>KNNPDPTIYPVLDWNDIKFQDVIGEGNFGQVLKARIKKDGLRMDAAIKRMKEYASKDDHRDFAGELEVLCKLGHHPNIINLLGACEHRGYLYLAIEYAPHGNLLDFLRKSRVLETDPAFAIANSTASTLSSQQLLHFAADVARGMDYLSQKQFIHRDLAARNILVGENYVAKIADFGLSRGQEVYVKKTMGRLPVRWMAIESLNYSVYTTNSDVWSYGVLLWEIVSLGGTPYCGMTCAELYEKLPQGYRLEKPLNCDDEVYDLMRQCWREKPYERPSFAQILVSLNRMLEERKTYVNTTLYEKF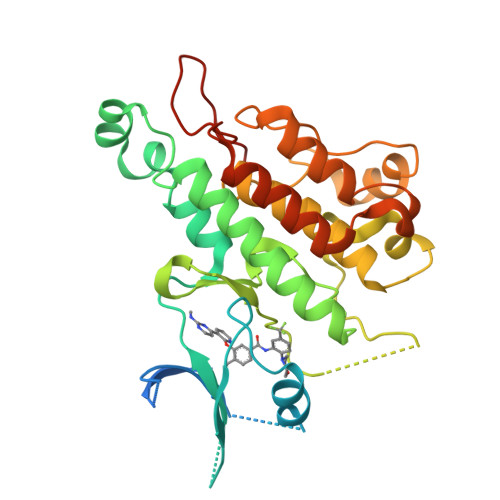TYAGIDCSAEEAA[2x]>[9x]AVTGQVDVKLNISTGCTVGGSQTEGNMNKFGTLNFGKTSGTWNNVLTAEVASAATGGNISVTCDGTDPVDFTVAIDGGERTDRTLKNTASADVVAYNVYRDAARTNLYVVNQPQQFTTVS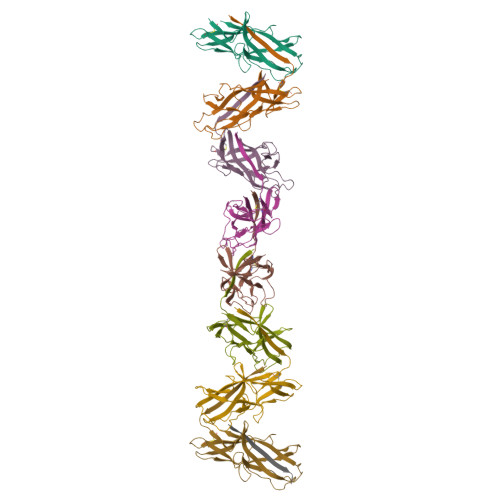GQATAVPIFGAIAPNTGTPKAQGDYKDTLLVTVNF>[2x]MQGVNIYNISAGTSVDL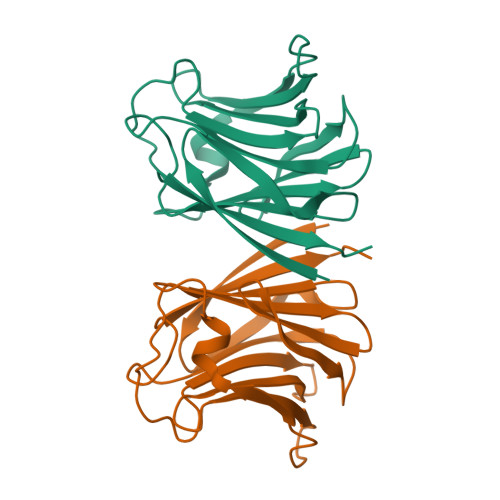AAPVTTGDGVTFFSSALNLNAGAGNPNNTTLNLFAENGAYLLHIAFRLQENVIIFNSRQPDGPWLVEQRVSDVANQFAGIDGKAMVTVFDHGDKYQVVINEKTVIQYTKQISGLTSSLSYNATEETSIFSTVVEAVTYTGLALEHHHHHH>GPVSWVCRFYQGKHRGVEVELPHGRCVFGSDPLQSDIVLSDSEIAPVHLVLMVDEEGIRLTDSAEPLLQEGLPVPLGTLLRA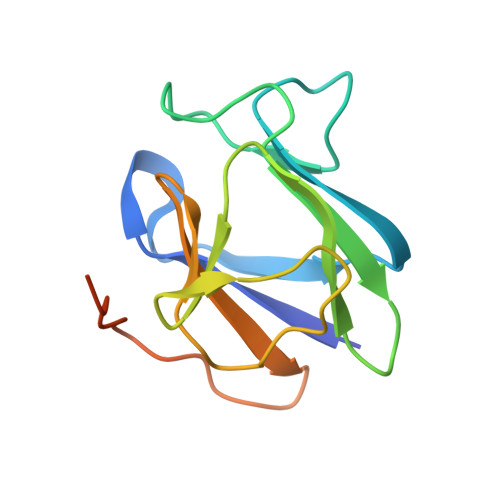GSCLEVGFLLWTFVAVGQPLPETLQVPTQRKEPTDRLPRSR[2x]(2S)-N-{(2S)-3-methoxy-1-[(naphthalen-1-ylmethyl)amino]-1-oxopropan-2-yl}-4-oxo-2-[(3-phenylpropanoyl)amino]-4-(1H-pyrrol-1-yl)butanamide 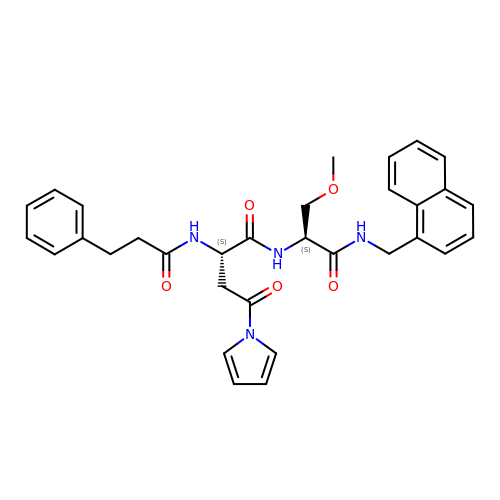(non-preferred name) | C32 H34 N4 O5 | MQUOXGJRURBMAU-NSOVKSMOSA-N> METPLDLLKLNLDERVYIKLRGARTLVGTLQAFDSHCNIVLSDAVETIYQLNNEELSESE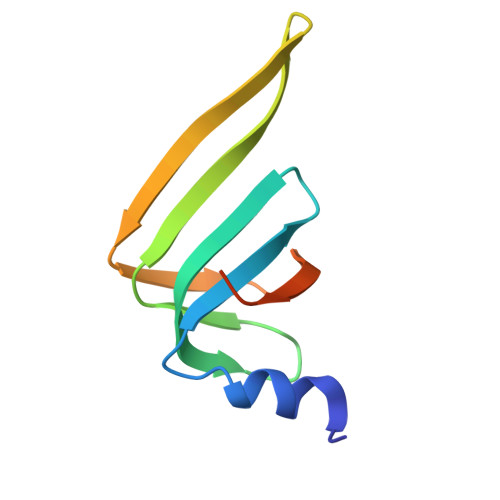RRCEMVFIRGDTVTLISTPSEDDDGAVEI>MPIIKEPIDFINKPESEAKKWGKEEEKRWFTKLNNLEEVAVNQLKNKEYKTKIDNFSTDILFSSLTAIEIMKEDENRNLFDVERIREALLKNTLDRDAIGYVNFTPKELGINFSIRDVELDRDISDETLDKVRQQIINQEYTKFSFISLGLNDNSINESVPVIVKTRVPTTFDYGVLNDKETVSLLLNQGFSIIPESAIITTIKGKDYILIEGSLSQELDFYNKGSEAWGAENYGDYISKLSHEQLGALEGYLHSDYKAINSYLRNNRVPNNDELNKKIELISSALSVKPIPQTLIAYRRVDGIPFDLPSDFSFDKKENGEIIADKQKLNEFIDKWTGKEIENLSFSSTSLKSTPSSFSKSRFIFRLRLSEGAIGAFIYGFSGFQDEQEILLNKNSTFKIFRITPITSIINRVTKM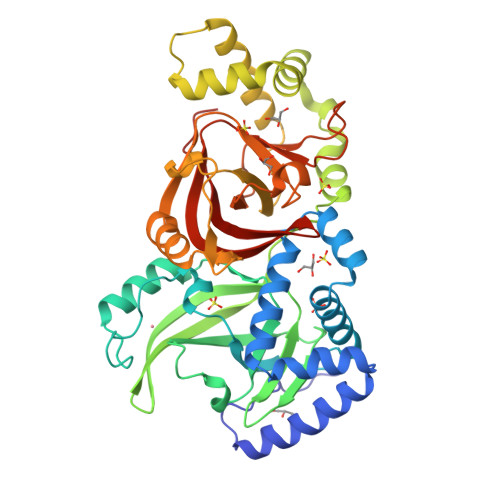TQVVIDAEGIQNKEI[6x]>MASTFRKSNVASTSYKRKVGPKPELTEDQKQEVREAFDLFDSDGSGTIDVKELKVAMRALGFEPRKEEMKKMISEVDKEATGKISFNDFLAVMTQKMAEKDTKEEILKAFRLFDDDETGKISFKNLKRVANELGE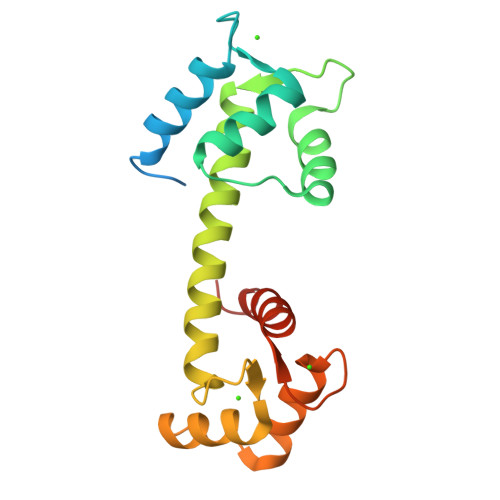SLTDEELQEMIDEADRDGDGEVNEEEFLKIMKKTNLYHHHHHH[2x]Neisserial adhesin A (NadA) is one of the main vaccine antigens, acts in host cell adhesion, and may influence colonization and invasion. NadA belongs to the OCA (oligomeric coiled-coil adhesin) family, a subgroup of the trimeric autotransporter adhesins (TAA), which generally mediate adhesion of Gram-negative bacteria to target cells or to the extracellular matrix and invasion. Similarly, recombinant NadA was reported to stimulate human monocytes by binding Hsp90 (26, 27). It was recently demonstrated that the NadA3 N-terminal region binds specifically to the endothelial cell receptor LOX-1 (low-density oxidized lipoprotein lectin-like receptor 1). The structure of NadA3 24–170 presents a small globular head region (residues 24 to 85) and a long trimeric coiled-coil motif made of canonical heptad repeats, plus the two novel undecad repeats.

We determined the crystal structure of NadA3 residues 24 to 170 using the molecular replacement approach and refined the structure to 2.45-Å resolution, with final Rwork and Rfree values of 20% and 22%. The asymmetric unit contained three copies of the polypeptide chain. Electron density maps revealed NadA3 residues 28 to 170. The structure presents the typical TAA family protein architecture; it is trimeric and elongated, with an N-terminal globular head. Despite sequence-based predictions that the NadA3 coiled-coil might be interrupted by other secondary structures in the region of residues 100 to 150 (23, 29, 30), the electron density maps of NadA3 24 to 170 display a continuous 160-Å-long coiled-coil stalk region extending from the head all the way to the C terminus. Within the head, NadA3 coordinates a chloride ion via the side chain of conserved residue N44, forming an N at the position d layer, similar to the observation about NadA5 (30). Two regions in NadA3 unexpectedly contain highly unusual 11-residue (undecad) repeat motifs wherein 11 amino acids form a coiled coil, deviating from the standard heptad repeat pattern. Intriguingly, the first undecad repeat spanning V97 to K107 presents an unusual d-e layer, previously identified in a few right-handed coiled coils and, to our knowledge, never detected before in undecads of left-handed coiled coils. The second undecad repeat, spanning L143 to F153, presents a more canonical hydrophobic d-a motif, comprised of residues L146 and G147. Nevertheless, superpositions of NadA3 and NadA5 reveal different positions of their wingtips by over 7 Å.

>[3x]ATNDDDVKKAATVAIAAAYNNGQEINGFKAGETIYDIDEDGTITKKDATAADVEADDFKGLGLKKVVTNLTKTVNENKQNVDAKVKAAESEIEKLTTKLADTDAALADTDAALDATTNALNKLGENITTFAEETKTNIVKIDEKLEAASKHHHHHH>[4x]SRSHQELISQLLQSYMKLLLPDDEKFHGGWALIDCDPSLIDATHRDVDVLLLLSNSAYYVAYYDDEVDKVNQYQRLSLENLEKIEIGPEPTLFGKPKFSCMRLHYRYKEASGY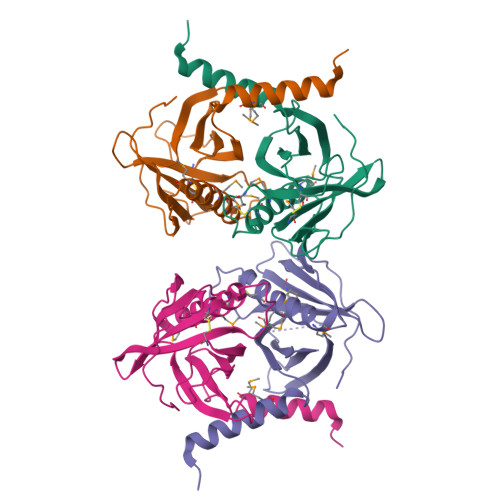FHTLRAVMRNPEEDGKDTLQCIAEMLQITKQAMGSDLPIIEKKLEAKASKPHEDII Here we show that Bdellovibrio bacteriovorus utilizes a small ankyrin repeat protein, Bd3460, to protect itself from endopeptidase activities during entry of prey. We demonstrate that endopeptidase complexation by Bd3460 prevents cell wall decrosslinking, and that both the Bd0816 and Bd3459 targets bind this self-protection protein via a common epitope. Previously, we assigned prey cell rounding to the action of two secreted Bdellovibrio peptidoglycan DD-endopeptidases, Bd0816 and Bd3459, that act to modify the invaded cell wall via hydrolysis of the structural 3-4 peptide crosslinks6. In summary, we conclude that we have identified and characterized the first ever self-protection protein encoded by predatory bacteria—ankyrin repeat protein Bd3460 from Bdellovibrio inhibits the prey wall decrosslinking enzymes Bd3459/Bd0816 and in doing so protects the predator from the shape transition that this catalyses in prey.

The structure is comprised of six sequential ankyrin repeats (AR1–AR6), which stack together to form the conventional ‘cupped hand' fold representative of ARPs, with the short β-strand ‘fingers' projecting out from the concave ‘palm'. The repeat regions largely conform to the 33 amino acid length of regular ARP motifs, with the longest loop present between AR3 and AR4 (sequence representation in Supplementary Fig. 7). The region surrounding the AR3:AR4 loop at the ‘centre' of Bd3460 displays three major deviations from the ankyrin structural consensus. Firstly amino acids V126 to G131 form an extended loop that differs from the usual tight turn present between the fingers of the other repeats of Bd3460/standard ARPs. Thirdly, the repeats of Bd3460 can be grouped such that AR1:4 and AR5:6 stack with a regular angular periodicity, but AR5 is twisted with respect to AR4. This 4+2 arrangement of repeats results in a partial cleft between these two subdomains, lined by D132, M136, A139, Q140, A167, A170 and V171. The cumulative effect of the three deviations from consensus structure is that the central AR3:AR4 loop projects further from the core of Bd3460 than the other loops, and at a relatively more acute angle. Bd3460 displays conformational sampling such that chains A to E adopt different relative flexation between AR4 and AR5.

>MKKSYLLAALIFFLAGLLHGTAFAMSGKSSKALNEAAEQGDLAKVKNLVQKNKIDLNAQDETGMTPLMNAAMGGNLDIVKFLLSKKVNLELKNNGGETALAFAVTNDAYDVAEELIKAGANVDIIVAGDEGDTLFMRAAQNNKKTAESILAKNKSLINKANTLGETALFAVARYGTPADIDFLIKKGADLKLKNKKGQTALDVAKEASNQDTAKALSKKKLEHHHHHHHH[5x]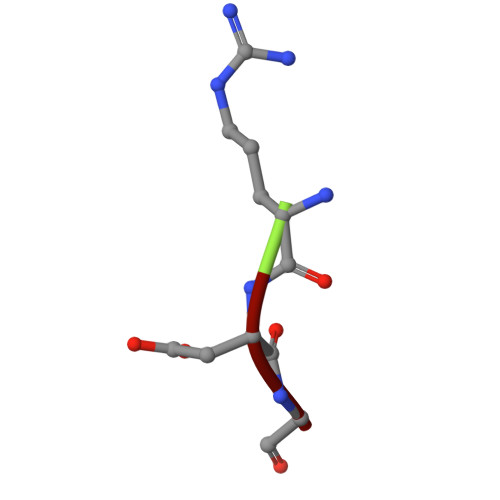> RDG>[2x]GPGSEFMDGPGASAVVVRVGIPDLQQTKCLRLDPTAPVWAAKQRVLCALNHSLQDALNYGLFQPPSRGRAGKFLDEERLLQDYPPNLDTPLPYLEFRYKRRVYAQNLIDDKQFAKLHTKANLKKFMDYVQLHSTDKVARLLDKGLDPNFHDPDSGECPLSLAAQLDNATDLLKVLRNGGAHLDFRTRDGLTAVHCATRQRNAGALTTLLDLGASPDYKDSRGLTPLYHSALGGGDARCCELLLHDHAQLGTTDENGWQEIHQACRFGHVQHLEHLLFYGANMGAQNASG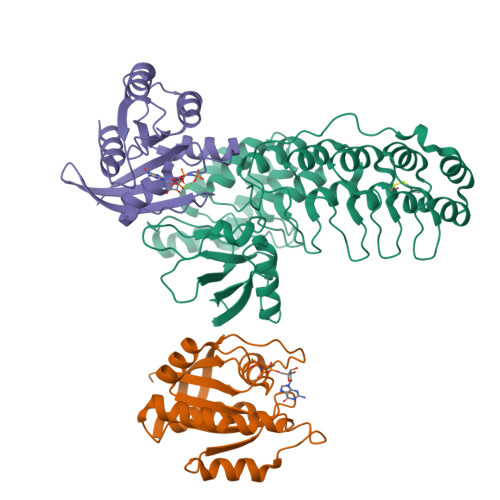NTALHICALYNQESCARVLLYRGANKDVRNYNSQTAFQVAIIAGNFELAEVIKTHKDSDVVPFRETPSYAKRRRLAGPSGLASPR;>[4x]GPHMREYKLVVLGSGGVGKSALTVQFVQGIFVEKYDPTIEDSYRKQVEVDAQQCMLEILDTAGTEQFTAMRDLYMKNGQGFALVYSITAQSTFNDLQDLREQILRVKDTDDVPMILVGNKCDLEDERVVGKEQGQNLARQWNNCAFLESSAKSKINVNEIFYDLVRQINR ATP13A2, which is mutated in juvenile-onset Parkinson’s disease and autosomal recessive spastic paraplegia 78, is a transporter with a critical role in balancing the polyamine concentration between the lysosome and the cytosol. The overall structure of hATP13A2 has a canonical P-type ATPase architecture, with the cytosolic A domain linking to TM1 and TM2 domains, and the N and P domains sitting on the TM4 and TM5. The P-type ATPases transport substrates by coupling ATP hydrolysis with protein phosphorylation states and adopting a series of intermediate states, consisting of E1, E1-ATP, E1P-ADP, E1P, E2P, E2-Pi, and E2, in a process known as the Post-Albers reaction. Here, we report seven cryo-EM structures of hATP13A2 in six intermediate states, importantly including the putative E2 and E1-like states, thereby providing a nearly complete atomic-level conformational cycle spanning the Post-Albers reaction process.

Although the E1 and E2 states are the two main conformations of the enzyme, the dynamic equilibrium between them makes it challenging to capture the structure of hATP13A2 in a single ATP/ADP-free state. Capturing the hATP13A2 structure in the E1-like state at 5.6 Å enabled us to assign the backbone of the amino acid sequence to the EM map. The structural comparison showed that hATP13A2 in the E1-like state presents a conformation similar to the E1-ATP structure, with the cytosolic domains next to each other. During the transition from the E1-like to E1-ATP state, the A domain, P-domain, and N-domain of hATP13A2 are tightly tethered together by ATP to form a catalytic center for ATP hydrolysis and aspartic acid phosphorylation. Four intermediate states (including E1-ATP, E1P-ADP, E2P, and E2-Pi) were solved at relatively high resolutions (3.2–3.7 Å), whereas the E1-like and putative E2 states were solved at medium resolutions (5.6 Å and 4.8 Å, respectively) probably due to the rapid dynamic equilibrium between the E1 and E2 states.

> RLSGYCGSPWRVIGYHVVVWMMAGIPLLLFRWKPLWGVRLRLRPCNLAHAETLVIEIRDKEDSSWQLFTVQVQTEAVSVGQLEPSPQSQAEDGRSQAAVGAVPEGAWKDTAQLHKSEEAKRVLRYYLFQGQRYIWIETQQAFYQVSLLDHGRSCDDVHRSRHGLSLQDQMVRKAIYGPNVISIPVKSYPQLLVDEALNPYYGFQAFSIALWLADHYYWYALCIFLISSISICLSLYKTRKQSQTLRDMVKLSMRVCVCRPGGEEEWVDSSELVPGDCLVLPQEGGLMPCDAALVAGECMVNESSLTGESIPVLKTALPEGLGPYCAETHRRHTLFCGTLILQARAYVGPHVLAVVTRTGFCTAKGGLVSSILHPRPINFKFYKHSMKFVAALSVLALLGTIYSIFILYRNRVPLNEIVIRALDLVTVVVPPALPAAMTVCTLYAQSRLRRQGIFCIHPLRINLGGKLQLVCFDKTGTLTEDGLDVMGVVPLKGQAFLPLVPEPRRLPVGPLLRALATCHALSRLQDTPVGDPMDLKMVESTGWVLEEEPAADSAFGTQVLAVMRPPLWEPQLQAMEEPPVPVSVLHRFPFSSALQRMSVVVAWPGATQPEAYVKGSPELVAGLCNPETVPTDFAQMLQSYTAAGYRVVALASKPLPTVPSLEAAQQLTRDTVEGDLSLLGLLVMRNLLKPQTTPVIQALRRTRIRAVMVTGDNLQTAVTVARGCGMVAPQEHLIIVHATHPERGQPASLEFLPMESPTAVNGVKDPDQAASYTVEPDPRSRHLALSGPTFGIIVKHFPKLLPKVLVQGTVFARMAPEQKTELVCELQKLQYCVGMCGDGANDCGALKAADVGISLSQAEASVVSPFTSSMASIECVPMVIREGRCSLDTSFSVFKYMALYSLTQFISVLILYTINTNLGDLQFLAIDLVITTTVAVLMSRTGPALVLGRVRPPGALLSVPVLSSLLLQMVLVTGVQLGGYFLTLAQPWFVPLNRTVAAPDNLPNYENTVVFSLSSFQYLILAAAVSKGAPFRRPLYTNVPFLVALALLSSVLVGLVLVPGLLQGPLALRNITDTGFKLLLLGLVTLNFVGAFMLESVLDQCLPACLRRLRPKRASKKRFKQLERELAEQR>[3x]MAQFDTEYQRLEASYSDSPPGEEDLLVHVAEGSKSPWHHIENLDLFFSRVYNLHQKNGFTCMLIGEIFELMQFLFVVAFTTFLVSCVDYDILFANKMVNHSLHPTEPVKVTLPDAFLPAQVCSARIQENGSLITILVIAGVFWIHRLIKFIYNICCYWEIHSFYLHALRIPMSALPYCTWQEVQARIVQTQKEHQICIHKRELTELDIYHRILRFQNYMVALVNKSLLPLRFRLPGLGEAVFFTRGLKYNFELILFWGPGSLFLNEWSLKAEYKRGGQRLELAQRLSNRILWIGIANFLLCPLILIWQILYAFFSYAE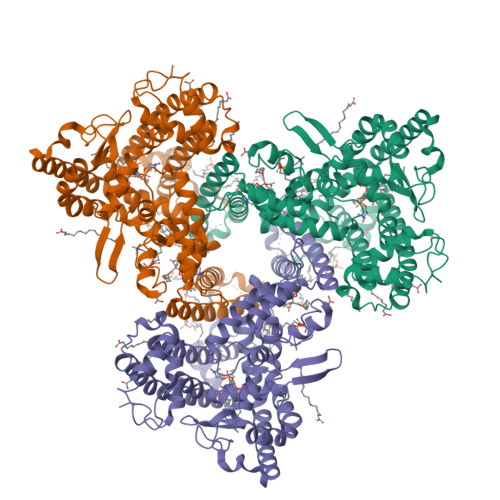VLKREPGALGARCWSLYGRCYLRHFNELEHELQSRLNRGYKPASKYMNCFLSPLLTLLAKNGAFFAGSILAVLIALTIYDEDVLAVEHVLTTVTLLGVTVTVCRSFIPDQHMVFCPEQLLRVILAHIHYMPDHWQGNAHRSQTRDEFAQLFQYKAVFILEELLSPIVTPLILIFCLRPRALEIIDFFRNFTVEVVGVGDTCSFAQMDVRQHGHPQWLSAGQTEASVYQQAEDGKTELSLMHFAITNPGWQPPRESTAFLG5-HEXYL-2-(4-NITROPHENOXY)PHENOL | C18 H21 N O4 | 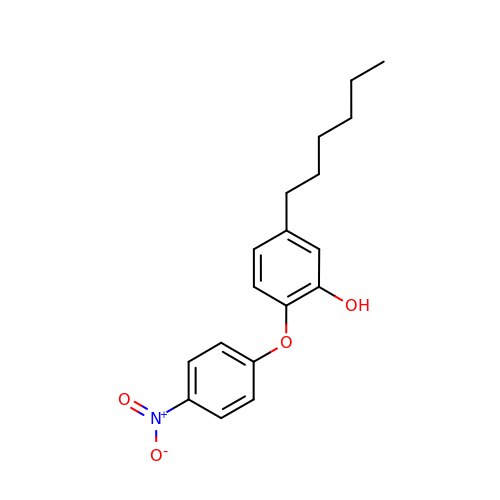NNNQXCYHIVPZRH-UHFFFAOYSA-N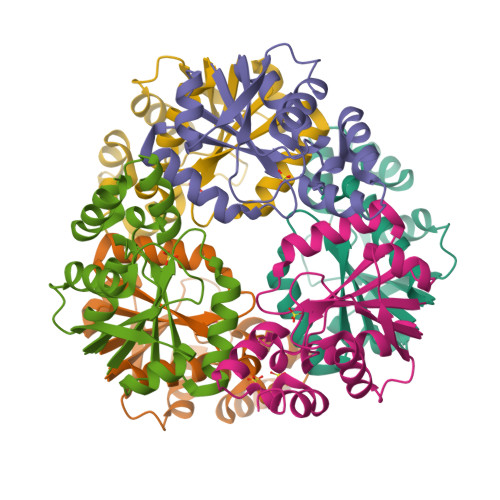>TGAVCPGSFDPVTLGHVDIFERAAAQFDEVVVAILVNPAKTGMFDLDERIAMVKESTTHLPNLRVQVGHGLVVDFVRSCGMTAIVKGLRTGTDFEYELQMAQMNKHIAGVDTFFVATAPRYSFVSSSLAKEVAMLGGDVSELLPEPVNRRLRDRLN[6x]(2R)-2,3-dihydroxypropyl ethyl hydrogen (S)-phosphate | C5 H13 O6 P | 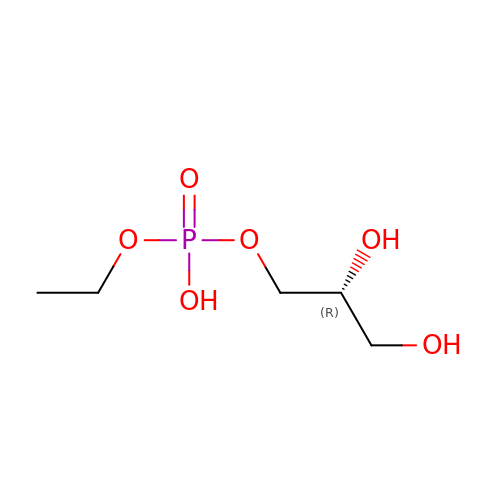DXARXEBAXKHIOU-RXMQYKEDSA-N>MSMYTTAQLLAANEQ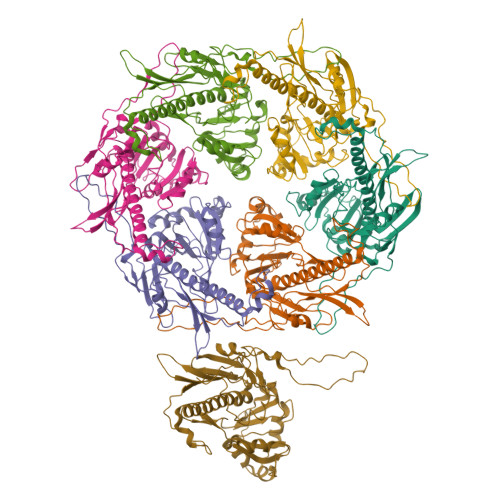KFKFDPLFLRLFFRESYPFTTEKVYLSQIPGLVNMALYVSPIVSGEVIRSRGGSTSEFTPGYVKPKHEVNPQMTLRRLPDEDPQNLADPAYRRRRIIMQNMRDEELAIAQVEEMQAVSAVLKGKYTMTGEAFDPVEVDMGRSEENNITQSGGTEWSKRDKSTYDPTDDIEAYALNASGVVNIIVFDPKGWALFRSFKAVKEKLDTRRGSNSELETAVKDLGKAVSYKGMYGDVAIVVYSGQYVENGVKKNFLPDNTMVLGNTQARGLRTYGCIQDADAQREGINASARYPKNWVTTGDPAREFTMIQSAPLMLLADPDEFVSVQLA[7x]>AGATHFLTPTGQASLVDDALYGWGADMLTVYLRCDPARLQALLPAGLKVADGLCMAYVGAFQSTSEDQPAAMLRNPAGAVYNEAALSIACTHGDRQGYFPAFVWVDKEWSLIRGWLNGYPKKIGAITLARPHPYNPVTGGLR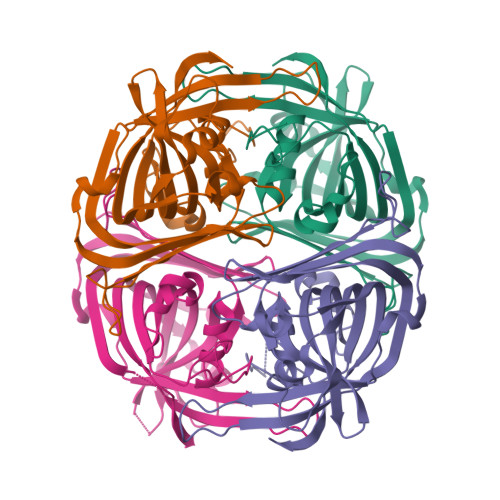EGAVVGGICARHGFTLFRLGLTVTRAGDAGDLRSRPATFGHRHWPALHPTQTPVSELVEVNRSDLRVGDIWAGEPFIELGSAPDEALECFADHEVLAGVTYSYGFRIGGATRLESL[4x]>[3x]EVYGIIAMQAAYRDYDSGDAKQDDNLGGMQLNNESRIGFRGKKQFANFEPTFIWQIEGGYVDPSFGGEGAGLGERDTFVGFESASWGQVRLGRVLTPMYELVDWPASNPGLGDVYDWGGAIGGAKYQDRQSNTIRWDSPMYADKFSIDAAVGAGDKAGLGAGDDYWGGIAAHYKLGPLQLDAAYEGNRNIEAEGQTWENNTYLVGVQGWFENGISFFAQYKYMEADASNGVNEKQDAMSAGLMYTTGDWQYKLGYAANFDLERDGKTLSNTSDDVVSAQIMYFVDPSAVLYARARMNDFNEGLDGLDDAARWTSGTNGDYNEYSVGVEYYF

VhChiP is a chitooligosaccharide-specific porin identified in the outer membrane of Vibrio campbellii type strain American Type Culture Collection BAA 1116. VhChiP contains three identical subunits, and in each subunit, the 19-amino acid N-terminal segment serves as a molecular plug (the “N-plug”) that controls the closed/open dynamics of the neighboring pores. VhChiP is a sugar-specific OM porin with the ability to selectively transport a range of chitooligosaccharides, chitohexaose being the most preferred. VhChiP consists of three identical β-barrels, each containing 16 β-strands connected on the extracellular side by eight hydrophilic loops and on the periplasmic side by eight short hydrophobic turns.

In this study, the crystal structures of VhChiP lacking the N-plug were determined in the absence and presence of chitohexaose. X-ray diffraction data of ligand-free truncated VhChiP were indexed, integrated, and scaled at a resolution of 2.40 Å in monoclinic space group C121, with a single trimer per asymmetric unit. The final model of the ligand-free truncated VhChiP was refined to Rwork and Rfree values of 18.0% and 22.6%, respectively. Inspection of the structures revealed that both truncated structures existed as intact trimers, indicating that the N-plug truncation did not affect the assembly of the protein. The crystal structures suggested that deletion of the N-plug did not interfere with trimer formation by VhChiP because the three subunits were held together by intramolecular L2–L2 interactions. The truncated channel inserted relatively quickly into the membrane and remained more stably open, with no gating. The average channel conductance of truncated VhChiP was 2.0 ± 0.4 nS, estimated from histogram analysis of 60 insertions, similar to that of WT VhChiP.> MKT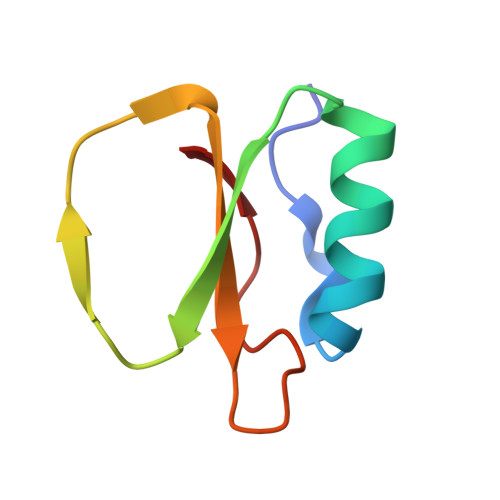EWPELVGKSVEEAKKVILQDKPAAQIIVLPVGTIVTMEARIDRVRLFVDRLDNIAQVPRVG> GPHMDAATLTYDTLRFAEFEDFPETSEPVWILGRKYSIFTEKDEILSDVASRLWFTYRKNFPAIGGTGPTSDTGWGCMLRCGQMIFAQALVCRHLGRDWRWTQRKRQPDSYFSVLNAFIDRKDSYYSIHQ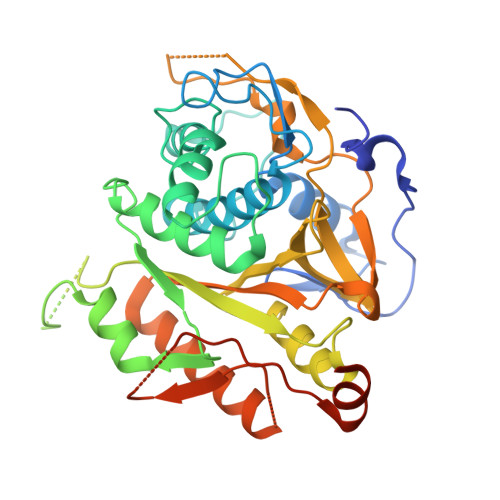IAQMGVGEGKSIGQWYGPNTVAQVLKKLAVFDTWSSLAVHIAMDNTVVMEEIRRLCRTSVPCAGATAFPADSDRHCNGFPAGAEVTNRPSPWRPLVLLIPLRLGLTDINEAYVETLKHCFMMPQSLGVIGGKPNSAHYFIGYVGEELIYLDPHTTQPAVEPTDGCFIPDESFHCQHPPCRMSIAELDPSIAVGFFCKTEDDFNDWCQQVKKLSLLGGALPMFELVEQQPSHLACPDVLNLSLDSSDVERLERFFDSEDEDFEILSL> MPDMANVESFDLDHTKVKAPYVRLAGVKTTPKGDQISKYDLRFLQPNQGAIDPAAIHTLEHLL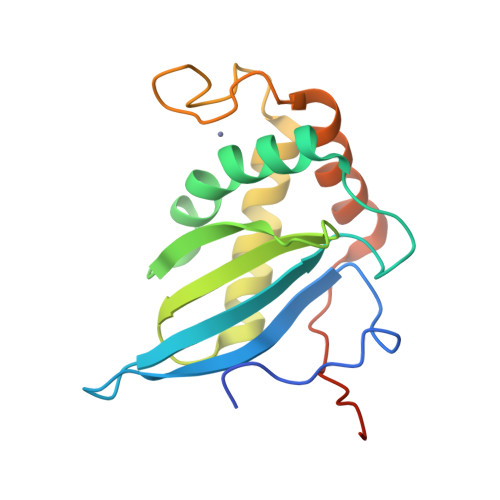AGYMRDHLEGVVDVSPMGCRTGMYMAVIGEPDEQGVMKAFEAALKDTAGHDQPIPGVSELECGNYRDHDLAAARQHARDVLDQGLKVQETILLERGSHHHHHH We isolated and characterized two Shigella podophages that have notably different features when compared with classical podophages and instead are most closely related to phage N4. We describe the isolation and characterization of phages Moo19 and B2, including whole-genome sequencing and analysis, cryo–electron microscopy (cryo-EM) structure determination, mass spectrometry, host range studies, and enzymatic assays of the tail proteins. Our work shows that these phages have divergent decoration proteins and unique tail structures, and encode and package their own phage-dependent RNA polymerase, and the tails, which display esterase activity, are dependent on specific O-antigen modifications of lipopolysaccharide (LPS) for entry. Moo19 and B2 are similar to bacteriophage N4—these are all T = 9 podophages, which encapsidate their own polymerases—a hallmark of this phage family.

We were able to clearly model several proteins with our C12-symmetrized maps including most residues for the portal proteins, tail adaptor proteins, and tail tubes for both Moo19 and B2. In addition, we were able to model the N-terminal residues of the tailspike proteins for both Moo19 and B2 but not the full-length proteins using the cryo-EM data as these are likely highly flexible at the linkage site. The portal shown in red was modeled from residues 17 to 675 of 760 total for Moo19 and residues 182 to 679 of 706 total for B2. The adaptor proteins were largely complete with all 234 residues modeled for Moo19 and residues 2 to 233 of 234 total for B2. Last, the tail tube shown in blue was modeled for residues 4 to 278 of 279 for Moo19 and residues 3 to 200 of 206 for B2. The tail tube of Moo19 (gp71) and the tail tube of B2 (gp34) both share a high sequence homology (>80%) with a number of phages that infect enteric hosts such as Shigella, Salmonella, Escherichia, Klebsiella, etc. In addition, Moo19 and B2 have C12 symmetry and not the proposed C15 symmetry of DEV. There is no homolog predicted in the genome, no similar protein seen in the mass spectrometry data, and no corresponding density observed in the B2 reconstruction. In G7C, this appendage is hypothesized to expand the host range; however, Moo19 and B2 have the same host range, so the function of gp81 in Moo19 is unclear at this time. Three major structural differences (see cartoon representation in Fig. 3B) include (i) the lack of the tail appendage, (ii) a single tailspike for Moo19 and a complex of two proteins for B2 (see next two paragraphs), and (iii) the completely different decoration proteins.

> MAKDELPIVNPEETGNLTDWDNEPTVSDLKSDYDSAYSSHSAQMSQITTWLNNLNVEGSAKPKKVPGRSSVQPMLIRKQAEWRYSALTEPFLSTDELFAVSPVTWEDREAAIQNQLVLNYQFNIKIDKVRFIDDYVRNAVNEGTVIVRVGWCNYTQMVKETVPVYAYYPAANEDQVAALQEALQLKLENPNAYNSLPDDIIASVDYSFENRGAFVAVQTGTEEVEYEKVIKNQPTVEVVNSQNVVIDPTCNGDISQAQFVIYSFETSKSDLEKDGRYKNLDKISASMSNPLNTPDHQVEDQSGFNFKDEPRKKFVAYEYWGWWDINGNGKTVPIVATFVGNTMIRLEENPFPDKKIPFVVVPYLPVPRSIYGEPDGALLEDNQKIIGATTRAMIDILARSANGQTGIRKDMLDVTNRRKFDKGEDYEFNANVDPRQGIYMHVSPEIPQSAPMMIQYQNNEAESLTGVKSFSQGIASQALGDVAAGIRGALDAASKRELGILRRLAQGVVEIGRKIISMNSEFLSEEEVVRVTNEQFVTVRRDELAGEFDLKLSISTAEADNQKAQELAFMLQTMGNSLPFEMSQMVLSDIARLRNMPDLAKRIESYQPQPDPLAQRKAELEIALLEAQIAETQSKAIENRASAGYKATQAQNVQSDTDLKNLDYVEQESGVKQARDVQKISAQAESQTQTKIVDYILKSGKPLSEI;> MKLSELFQMLSVGELSLIRTGNDGQGIRTQDYPKVIAQLNAGLTNLHARFPLLEKEVIIQQYEQISKYYLRSEFAQMNTTSTEKYKYLMDSPTERFLDDVIRVERVFDECGCPLYLNNEPCCGSIVTPSFDCIQIVYPIETNALFVTYRANHPKIALTTTDLNTEVRIPASHEKALTYYIASQLYSNSPNPETAAKGVEWSQRFEAECTKIENLDLDNAHIAQTNVKPEMRGWV;> MAVVIEPITNEDLTTKVVDGTGIFDELMTAANAHLSAQWDMERITGTQYAEVYLGQLTAVLQQAVTFLIEKDKTYLNNLLINAQIELANKQIELADKELEKADKEIELLELNKELIAQKVKTEKAQISDTVDSVPVTGIIGAQIALYKQQKDGFIRDAEQKALKIISDTWITRKTVDDGTPLPTGFDTAAVDAFTRKVADGVSVNY;>[3x]MIRTTNTCCGNQAGMVEKFIGTAYDVVKTVYDNLGEIQFIYNFLNDYGVLITVDSVTELQELPTTAKYTRVYSSTPTGVRIYTDYLYVEGDRTGVLPSDPTATGSWVVVGSSNSGAATGTGAYIPFVFNNGSAAGGETTIVVPDYTIGVPEIYVEGFRQQVGRGFTFNSVNLTVTLAQPLEQGDEVVLMLSGNPAVPDNPNIDSWTVINWIYNNGAAVGGEQVIVIPYTFQTVPAIFKNGLRYQGGLSTQSYTVDQDNKRILLTEPLSTNDRLVVQLGGELVTLESPDRSLYEIARATNMKDSEVIKSDNTVETLNGKRILYDIVSQVYYWIPSSVPNNVYIQSVVNGQLTYLPGNIVVTLTPIVTLGLSGTTAQRPIGVLTGTQHFDTTLGKPIWFNGTAWVDSTGAVV> KETAAAKFERQHMDS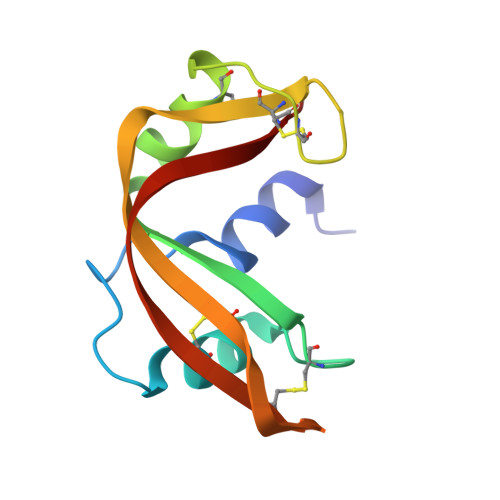STSAASSSNYCNQMMKSRNLTKDRCKPVNTFVHESLADVQAVCSQKNVACKNGQTNCYQSYSTMSITDCRETGSSKYPNCAYKTTQANKHIIVACEG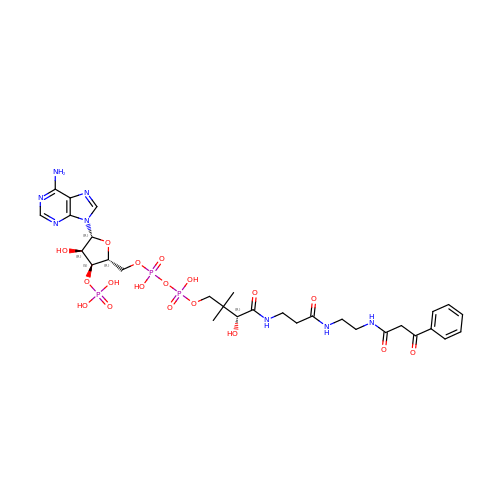[(2R,3S,4R,5R)-5-(6-amino-9H-purin-9-yl)-4-hydroxy-3-(phosphonooxy)oxolan-2-yl]methyl (3R)-3-hydroxy-2,2-dimethyl-4-oxo-4-[(3-oxo-3-{[2-(3-oxo-3-phenylpropanamido)ethyl]amino}propyl)amino]butyl dihydrogen diphosphate | C30 H43 N8 O18 P3 | DMKCDUQHKCJISD-FUEUKBNZSA-N>[2x]GTLDTTWKEATLPQVKAMLEKDTGKVSGDTVTYSGKTVHVVAAAVLPGFPFPSFEVHDKKNPTLEIPAGATVDVTFINTNKGFGHSFDITKKGPPYAVMPVIDPIVAGTG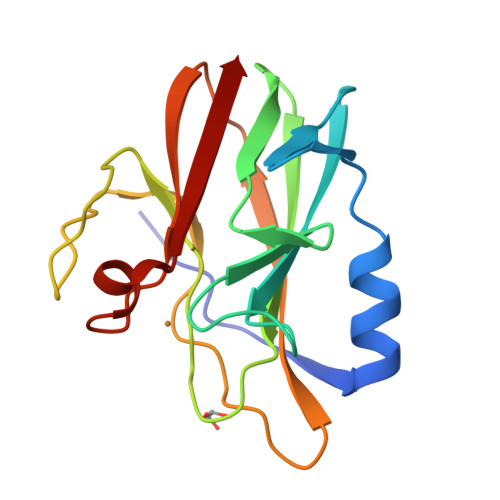FSPVPKDGKFGYTNFTWHPTAGTYYYVCQIPGHAATGLFGKIVVK>SNAMSEKPTSIKLVVVGDGAVGKTCLLISYSIRKFPEDYIPTVFDNYVVSLTAGTRQIQLALWDTAGLEEYDQLRPLSYSSASIFLICFSVTSSVSYDNVITKWHPEVIHFAPKVPIILVGTKLDTRNDPAIVKRLTEQGMTVINTA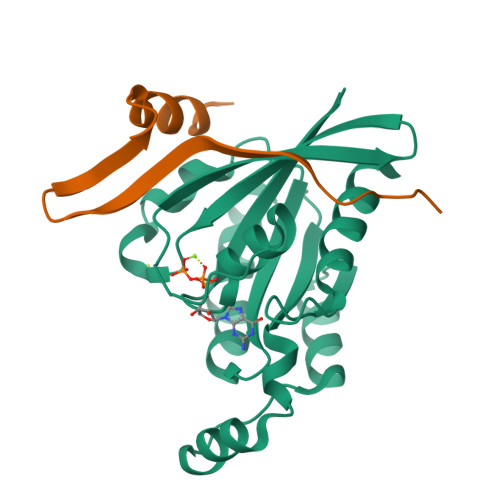KGEELKNRIKAVKYIECSAKTSENLKTVFDEAVKTVLMN[4x];>SNAELIISDPTDFEQITHVELGDSGLTGFPPEWREKLIKAGLTEAEINTNEDSAKLVAASGISNDNGNRT[4x]>[2x]MG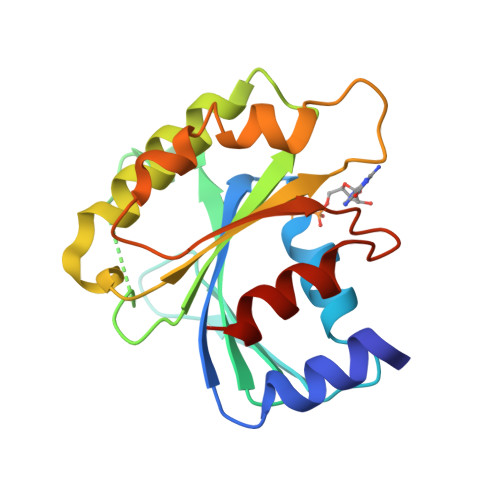ILFTRIWRLFNHQEHKVIIVGLDNAGKTTILYQFSMNEVVHTSPTIGSNVEEIVINNTRFLMWDIGGQESLRSSWNTYYTNTEFVIVVVDSTDRERISVTREELYKMLAHEDLRKAGLLIFANKQDVKECMTVAEISQFLKLTSIKDHQWHIQACCALTGEGLCQGLEWMMSRLKIR>[4x]MGSSHHHHHHMALLQKTRIINSMLQAAAGKPVNFKEMAETLRDVIDSNIFVVSRRGKLLGYSINQQIENDRMKKMLEDRQFPEEYTKNLFNVPETSSNLDINSEYTAFPVENRDLFQ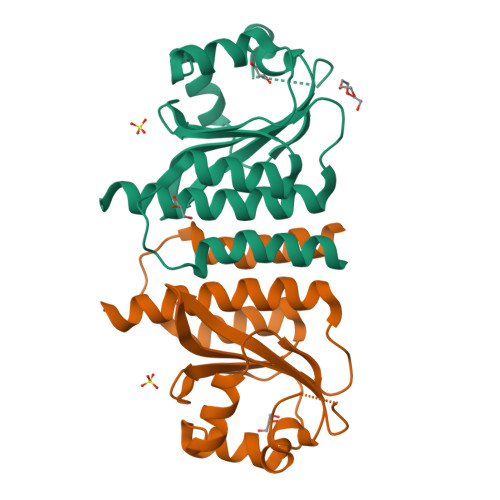AGLTTIVPIIGGGERLGTLILSRLQDQFNDDDLILAEYGATVVGMEILREKAE>SNAMAEDKGRKVVVSALQFACTDDVSTNVTTAERLVRAAHKQGANIVLIQELFEGYYFCQAQREDFIQRAKPYKDHPTIMRLQKLAKELGVVIPVSFFEEANNAHYNSIAIIDADGTDLGIYRKSHIPDGPGYEEKFYFNPGDTGFKVFQTKYAKIGVAICWDQWFPEAARAMALQGAEILFYPTAIGSEPHDQSIDSRDHWKRVMQGHAGANLVPLVASNRIGNEIIETEHGKSEIKFYGNSFIAGPTGEIVSIADDKEEAVLIAEFNLDKIKSMRHCWGVF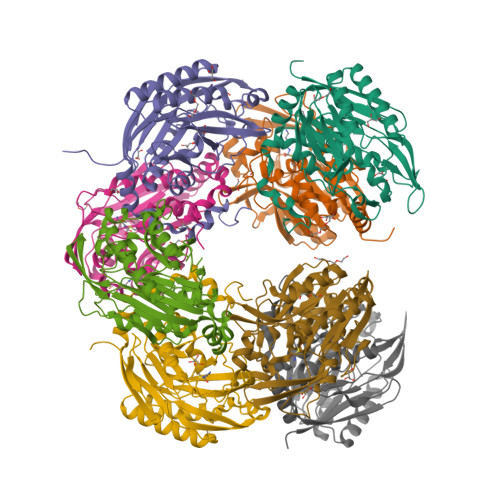RDRRPDLYKVLLTLDGKNPVL[16x]>[2x]MASQPNSSAKKKEEKG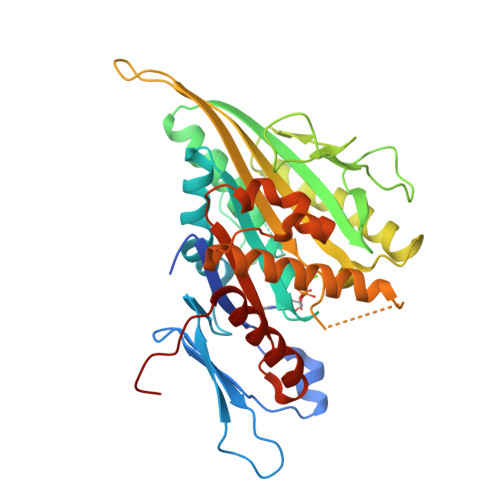KNIQVVVRCRPFNLAERKASAHSIVECDPVRKEVSVRTGGLADKSSRKTYTFDMVFGASTKQIDVYRSVVCPILDEVIMGYNCTIFAYGQTGTGKTFTMEGERSPNEEYTWEEDPLAGIIPRTLHQIFEKLTDNGTEFSVKVSLLEIYNEELFDLLNPSSDVSERLQMFDDPRNKRGVIIKGLEEITVHNKDEVYQILEKGAAKRTTAATLMNAFSSRSHSVFSVTIHMKETTIDGEELVKIGKLNLVDLAGSENIGRSGAVDKRAREAGNINQSLLTLGRVITALVERTPHVPYRESKLTRILQDSLGGRTRTSIIATISPASLNLEETLSTLEYAHRAKNILNKPEVNQKL>MGSSHHHHHHSSGIREEEFVNNPQGNFEQLWKIIDEQYCFLDYKQIDWDEIHTRYQKLITPNMGSEGLFEVLSE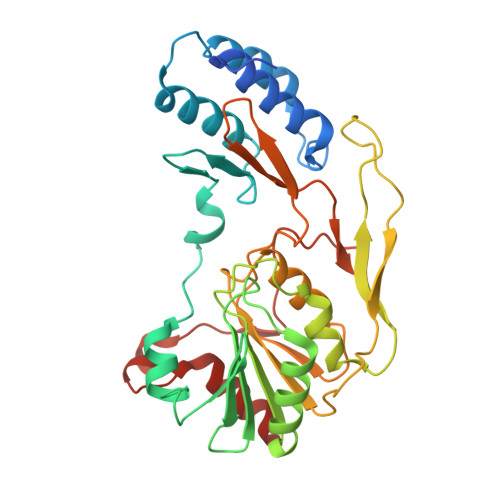MLYELQDGHVNLASAHNVSYYDAWYQDYPRNFRADLLEDSYLGRASTDYRTAAGLKYKILKDNIGYIRYESFADPVGNGNLDEVLSYLSVCNGLIIDVRDNGGGNATNSARIASRFTNEKILTGYISHKTGTGHNDFSKPYAIYLEPANGVRWQKKVVVLTNRRSFSATNDFVNHMRCLPNVTTIGDKTGGGSGMPFTSELPNGWSVRFSASPHFDAEMNHIEFGIEPDIKADMLQEDELRGKDTLIEMARKLLSE[2x]>[4x]SYYSTLQCRNNHGHCRRLCFHGEQWIGNCNGRHQHCCK

Defensins, a family of cysteine-rich cationic host defence peptides, are a major component of the innate immune systems of all plant and animal species, however crocodilian defensins are poorly characterised. We now report the functional and structural characterisation of Crocodylus porosus β-defensin 13 (CpoBD13). We now show that the saltwater crocodile defensin CpoBD13 harbors potent antifungal activity that is mediated by a pH-dependent membrane-targeting action. CpoBD13 binds the phospholipid phosphatidic acid (PA) to form a large helical oligomeric complex, with specific histidine residues mediating PA binding.

Consequently, we determined the structure of a CpoBD13:PA complex, which was refined to a resolution of 1.45 Å. The asymmetric unit features four CpoBD13 protomers and four PA molecules. Examination of the mode of engagement of PA with the different CpoBD13 chains revealed the presence of two different PA binding sites. In contrast, the type I site features contributions from three different CpoBD13 chains. N30 from chain A and H21 from chain B contact the phosphate of the PA headgroup. Furthermore, the crystallographic symmetry mate of chain B (denoted as B’) also contributes via R9 binding to the PA headgroup. Three additional contacts are formed by S1 from chain A, which forms hydrogen bonds with two oxygen atoms in the acyl chains of PA and the linking oxygen with the phosphate headgroup. The type II site involves contacts of R17 and H35 with the phosphate of the PA headgroup. An additional contact is formed with N28 and a carboxyl group of the acyl chain. Intriguingly, the structure of our CpoBD13:PA complex revealed the existence of large and continuous helical oligomers.> MSGMIKVPEDLERIGRELRARGLDTK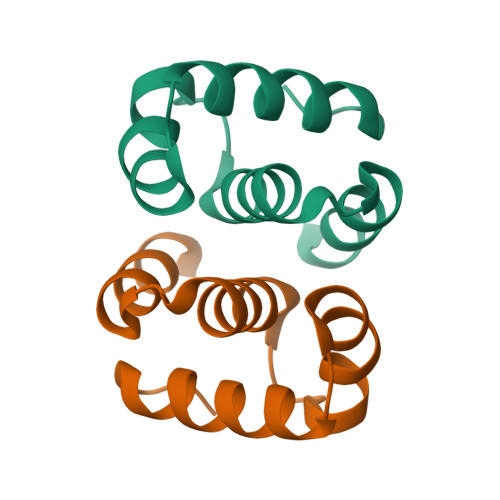RLLEEGPKLYPELSIPDLMAIALYDHLNLDPEFLYRLLQQSRGS>[4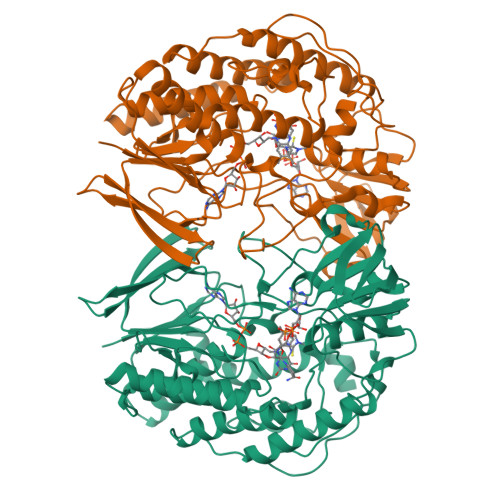x]MTKRVAVIGAGPSGLAQLRAFQSAADQGAEIPEIVCFEKQANWGGLWNYTWRTGLDENGEPVHCSMYRYLWSNGPKEGLEFADYSFEEHFGKQIASYPPRAVLFDYIEGRVHKADVRKWIRFNSPVRWVSYDAETAKFTVTAHNHETDSTYSAAFDHVICASGHFSTPNVPFYEGFDTFNGRIVHAHDFRDAREFEGKDVLVMGASSSAEDIGSQCWKYGAKSITSCYRSAPMGYAWPDNWEEKPALEKLTGKTAHFADGSTRDVDAIILCTGYKHFFSFLPDDLRLKTANRLATADLYKGVAYVHNPAMFYLGMQDQWFTFNMFDAQAWWVRDAILGRITLPKDKAAMLADVAERETREEASDDVKYAIRYQADYVKELVAETDYPSFDIDGACDAFFEWKKHKAKDIMAFRDNSYKSVITGTMAPVHHTPWKEALDDSMEAYLQNHHHHHH> GP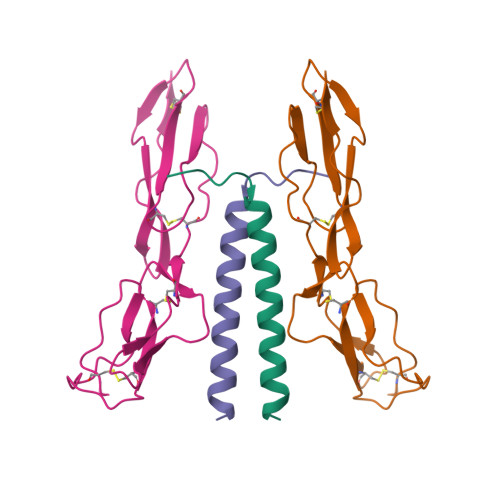GSNSKNPVPVKKEAKLSEAELHDKIAALEEEKAELFEKLDKVEEEHKKVEEEHKKDHEKLEKKSEDVERHYLRQLDQEYKEQQERQKNLEELERQSQREVEK;> GPGSNCGPPPTLSFAAPMDITLTETRFKTGTTLKYTCLPGYVRSHSTQTLTCNSDGEWVYNTFCIYKRCRHPGELRNGQVEIKTDLSFGSQIEFSCSEGFFLIGSTTSRCEVQDRGVGWSHPLPQCEI>MEDGAQMRVVAFGDQTYDCSEAVSQLLRVRDDAIVVDFLERAPAVLKAELARLSSEQQEETPRFATLAELVPRYRAGTLNPAVSQALTCIAQLGLFIRQHSSGQEAYPTAHDSCITGVCTGALTAVAVGSASSVTALVPLALHTVAVAVRLGARAWEIGSCLADARRGANGRYASWTSAVGGISPQDLQDRISAYTAEQALASVSVPYLSAAVGPGQSSVSAAPVILDAFLSTLLRPLTTTRLPITAPYHAPHLFTAKDVQHVTDCLPPSEAWPTVRIPIISFSRDEAVSRGASFPAAMSEAVRDCLIRPIALDRMAVSIANHARDLGKDSVLPSPIALSFSDKLGPQVNSHLPGAKAPTPELTSKSIPSAIGAEQQPMAKSPIAILAASGRFPQSSSMDQFWDVLINGVDTHELVPPTRWNAATHVSEDPKAKNVSGTGFGCWLHEAGEFDAAYFNMSPREAPQVDPAQRLALLTATEALEQAGVVPNRTSSTQKNRVGVWYGATSNDWMETNSAQNVDTYFIPGGNRAFIPGRVNYFHKFSGPSYTIDTACSSSLAALHMACNALWRGEVDTAIVGGTNVLTNPDMTAGLDAGHFLSRSGNCKTFDDEADGYCRGEAVVTLILKRLPDAQADKDPIQASILGIATNHSAEAASITRPHAGAQQDLFQQVLTETGLTANDISVCEMAGTGTQAGDSGETTSVVETLAPLNRSGSAVRTTPLYIGAVKSNVGHAESAAGVSSLAKILLMLKHSKIPPHVGIKTKLNHRLPDLAARNTHIARSEVPWPRPKNGKRRVLLNNFSAAGGNTCLVLEDAPEPEDSQEVDPREHHIVALSAKTPDSMVNNLTNMITWIDKHSGDSLATLPQLSYTTTARRVHHRHRAVATGTDLLQIRSSLQEQLDRRVSGERSIPHPPNGPSFVLAFTGQGSAFAGMGVDLYKRFASFRSDIARYDQICEGMSLPSIKAMFEDEKVFSTASPTLQQLTHVCFQMALYRLWKSLGVQAKAVVGHALGEYAALYAAGVLSQSDTLYLVGRRAQLMEKHLSQGTHAMLAVRAKEEAIVAAIDGPPGEAYEFSCRNGEQRNVLGGTVAQIQAAKA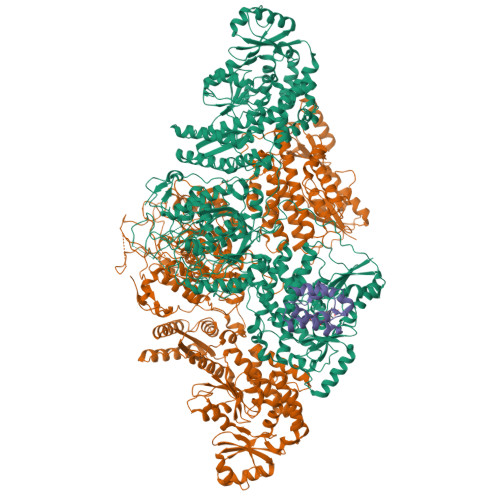ALEAKKIRCQYLDTPMAFHTGQVDPILPELLQVAAACSIQDPQIPVISPAYGKVIRSAKDFQPEYFTHHCRSSVNMVDALQSAVEEGLLDKNVIGLEIGPGPVVTQFVKEAVGTTMQTFASINKDKDTWQLMTQALAKFYLAGASVEWSRYHEDFPGAQKVLELPAYGWALKNYWLQYVNDWSLRKGDPAVVVAASAAALEHHHHHH[2x];> GSHMDPSPNEIGTVWRDALKILSEESGLTDEELTDDTSFADVGVDSLMSLVITSRLRDELDIDFPDRALFEECQTIFDLRKRFSGSTE> MGSYLHEPPGDEPSMRIEQPKTADRAPEQVAIHICEPSKVVTESFPFSETAEPEAKSKNCPCPEIARIGPCPNKPPKIPINRGLSRISTNKSRPKSRFGEPSWPVESSLDLTSQSPVSPYREEAFSVENCGTAGSRRGSFARGTTSRAASSSRKDETKEGPDEKEVYQRVTAQLSARNQKRMTVKLMIELSVFLCLLGCLVCSLTV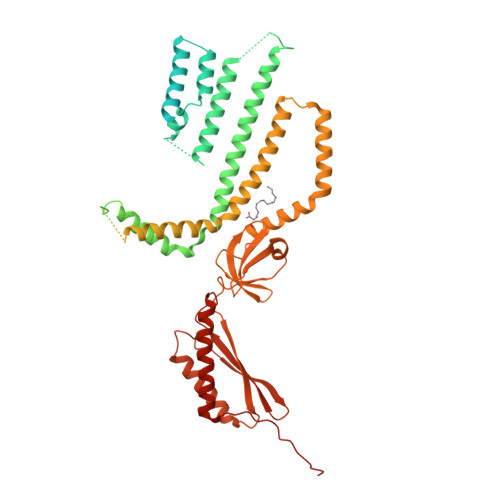DGFKRYTVIGLDIWKWFLLLLVIFSGMLITHWIVHVAVFFVEWKFLMRKNVLYFTHGLKTSVEVFIWITVVLATWVMLIKPDVNQPHQTRKILEFVTWTIVTVLIGAFLWLVKTTLLKILASSFHLNRFFDRIQESVFHHSVLQTLAGRPVVELAQGISRTESQDGAGQVSFMEHTKTQNKKVVDVGKLHQMKQEKVPAWTMQLLVDVVSNSGLSTMSGMLDEDMVEGGVELDDDEITNEEQAIATAVRIFDNIVQDKVDQSYIDRVDLHRFLIWEEVDHLFPLFEVNEKGQISLKAFAKWVVKVYNDQAALKHALNDNKTAVKQLNKLVTAILIVMMIVIWLIVTGIATTKLIVLLSSQLVVAAFIFGNTCKTIFEAIIFVFVMHPFDVGDRCVIDGNKMLVEEMNILTTVFLKWDKEKVYYPNSILCTKAIGNFFRSPDQGDVLEFSVDFTTPVLKIGDLKDRIKMYLEQNLNFWHPQHNMVVKEIENVNKIKMALFVNHTINFQDFAEKNRRRSELVLELKKIFEELDIKYNLLPQEISIRNMGSGSLEVLFQ>MAHHHHHHMLTNWNYQLTHFVTSAPD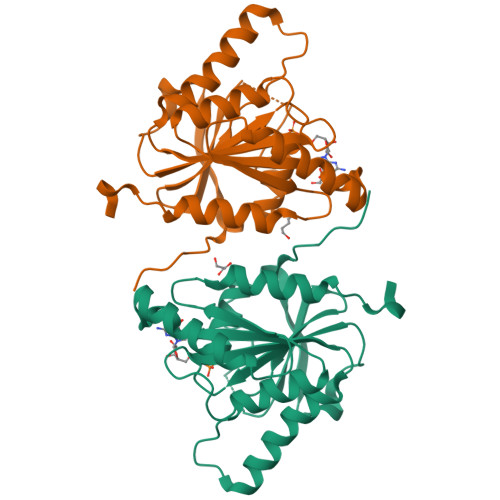IRHLPADTGIEVAFAGRSNAGKSSALNTLTNQKNLARTSKTPGRTQLINLFEVAEGKRLVDLPGYGYAQVPEEMKIKWQRALGEYLEKRLCLKGLVVLMDIRHPLKDLDQQMIEWAVESDIQVLVLLTKADKLASGARKAQVNMVREAVLAFNGDVQVEPFSSLKKSGVDKLRQKLDSWFNEIPPQEAVEDAE[2x]> MAHHHHHHMSPDSNTDNSRPGVSSSEIPRTDTERKT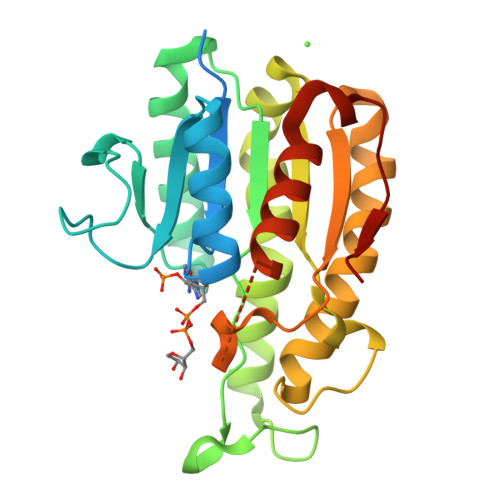LVLTGASRGIGHATVKRFSLAGWRVITCSRQDFSENCPWPAGPEDHIKVDLSDPEDIGKAIAEIRRRLEANGSKLHALVNNAGISPKAEGGRRMNSIETPMAVWRDVFQVNFMAPIMLARGLFKELEAAQGSVVNVTSIAGSRVHPFAGTAYATSKAALAALTREMASDFGPYGIRVNAIAPGEIDTAILSPGTDKLVEQLPMRRLGKTSEVAETIYFLCTETSSYVTGSEIHINGGQHV4-ethyl-5-methyl-2-(1H-tetrazol-5-yl)-1,2-dihydro-3H-pyrazol-3-one 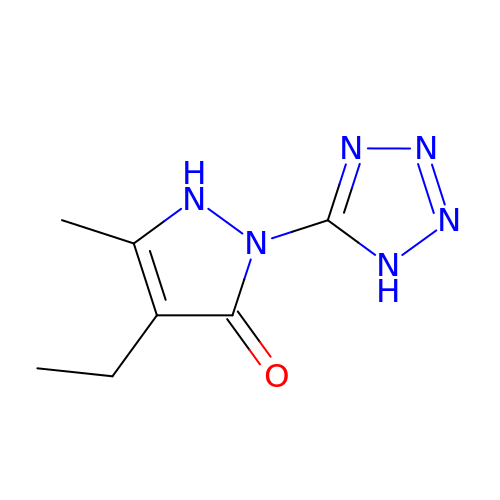| C7 H10 N6 O | WAVWUEFMWJZZFB-UHFFFAOYSA-N>[8x]MSCINLPTVLPGSPSKTRGQIQVILGPMFSGKSTELMRRVRRFQIAQYKCLVIKYAKDTRYSSSF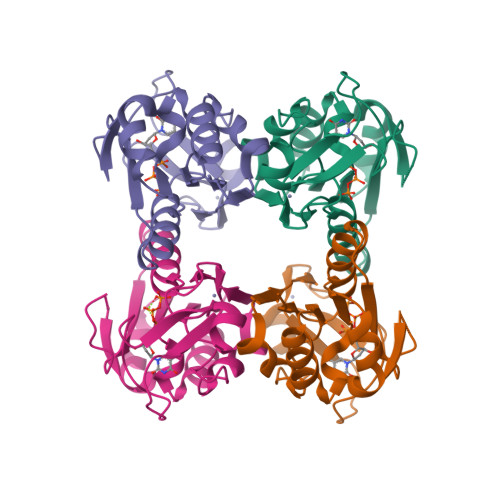CTHDRNTMEALPACLLRDVAQEALGVAVIGIDEGQFFPDIVEFCEAMANAGKTVIVAALDGTFQRKPFGAILNLVPLAESVVKLTAVCMECFREAAYSKRLGTEKEVEVIGGADKYHSVCRLCYFKKA>[8x]GSFVGSIDQGTTSSRFLIFNGEGNPVASHQIEFENLYPKSGWHEQDPYELLNSVQQCIDGAMHKFASLGYSKENIRAIGITNQRETTVVWDSVTGEPLHNAIVWPDTRTSALVRELKARQSADSLLELCGLPLSTYPSSVKLLWLIQNVDAVKQAYEEGRLAFGTVDSWLIYKLNGGAQAERPIHVTDSTNASRTMFMNLRTLQYDDKLLGFFGIDRNKIKLPKIVPSSDPEAFGKVATGALAGVPIAGCLGDQSSALVGQCGFSPGQAKNTYGTGCFLLYNVGTEPVISKYGLLATVAYDFGRGRKPVYALEGSIAVAGAGITFLMNNLGFAPKPSEINALAESVLDNGGVVFVTAFSGLFAPYWIDDAKGTLFGITQHTTKGHIARATLEATCYQTRAILDAMEKDSGHKLESLAVDGGLSASDLCMQTQADISGIPVDRPRMRETTALGAAIAAGLATGVWRELDHVKESIAGGANGNGKKN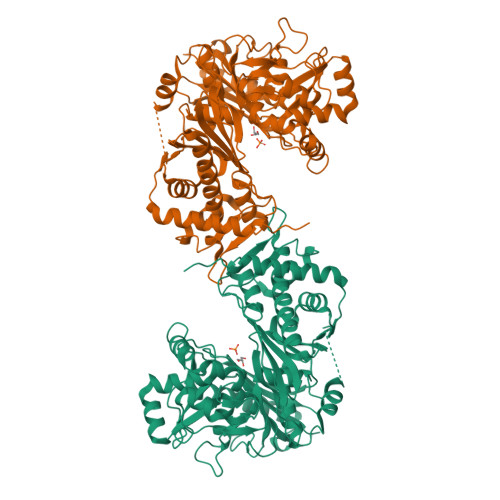AREVFYPKMDRKKAERLFRKWEQAVEMSRGWVREQEEEDGE>GHMAAAAELSLLEKSLGLSKGNKYSAQGERQIPVLQTNNGPSLTGLTTIAAHLVKQANKEYLLGSTAEEK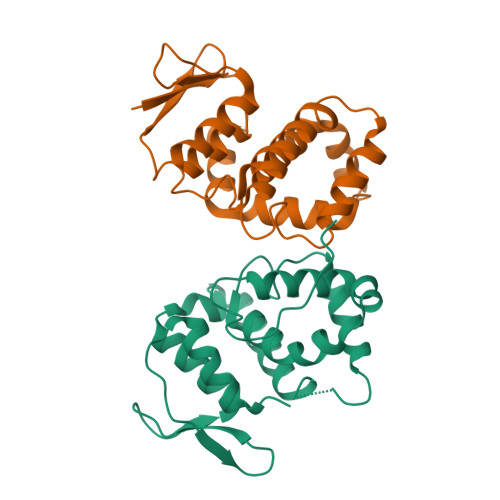AIVQQWLEYRVTQVDGHSSKNDIHTLLKDLNSYLEDKVYLTGYNFTLADILLYYGLHRFIVDLTVQEKEKYLNVSRWFCHIQHYPGIRQHLSSVVFIKNRL[4x];>[4x]MATLSLTVNSGDPPLGALLAVEHVKDDVSISVEEGKENILHVSENVIFTDVNSILRYLARVATTAGLYGSNLMEHTEIDHWLEFSATKLSSSDSFTSTINELNHSLSLRTYLVGNSLSLADLSVWATLKGNAAWQEQLKQKKAPVHVKRWFGFLEAQQAFQSVGTKWDVSTTKAR> MHHHHHHLVPRGSMLDFEKPLFEIRNKIESLKESQDKNDVDLQEEIDMLEASLERETKKIYTNLKPWDRVQIARLQERPTTLDYIPYIFDSFMELHGDRNFRDDPAMIGGIGFLNGRAVTVIGQQRGKDTKDNI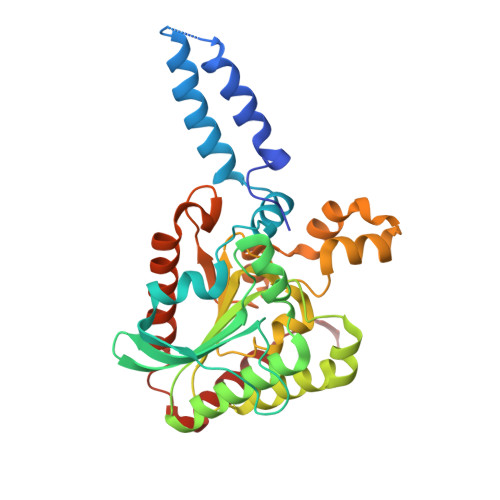YRNFGMAHPEGYRKALRLMKQAEKFNRPIFTFIDTKGAYPGKAAEERGQSESIATNLIEMASLKVPVIAIVIGEGGSGGALGIGIANKVLMLENSTYSVISPEGAAALLWKDSNLAKIAAETMKITAHDIKQLGIIDDVISEPLGGAHKDIEQQALAIKSAFVAQLDSLESLSRDEIANDRFEKFRNIGSYIE>CCGATATCGG[2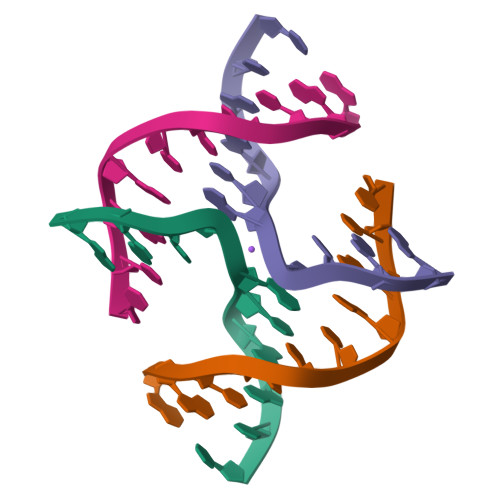x]> GDSFYIRTHFEYEKESPYGLSFNKGEVFRVVDTLYNGKLGSWLAIRIGKNHKEVERGIIPNKNRAEQLASVQYVQTKFPAYERVVLREAGFLRPVTIFGPIADVAREKLAREEPDIYQIAKSEPRDAGTDQRSSGIIRLHTIKQIIDQDKHALLDVTPNAVDRLNYAQWYPIVVFLNPDSKQGVKTMRMRLCPESRKSAR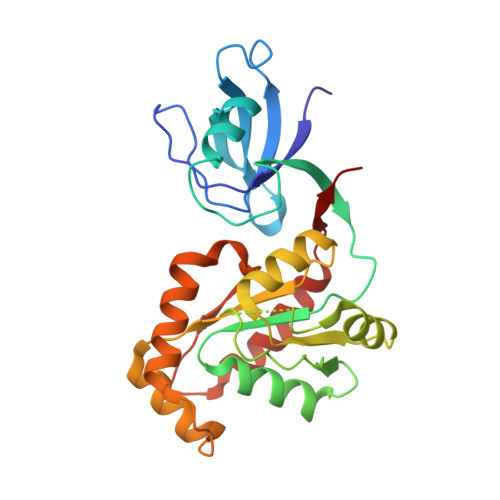KLYERSHKLRKNNHHLFTTTINLNSMNDGWYGALKEAIQQQQNQLVWVSEG>[2x]GMLKSKIKEEYVQM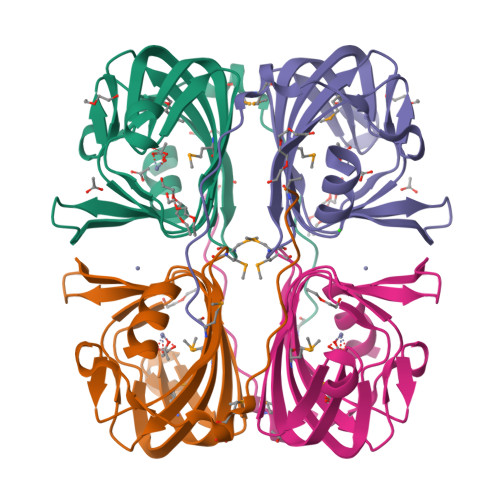DQVDWKPFPAAFSTGGIRWKLLHVSPEMGSWTAIFDCPAGSSFAAHVHVGPGEYFLTKGKMDVRGGKAAGGDTAIAPGYGYESANARHDKTEFPVASEFYMSFLGPLTFVKPDGSPIAVIGWEDAQGAWAA>[2x]PGMAGDSEQTLQNHQQPNGGEPFLIGVSGGTASGKSSVCAKIVQLLGQNEVDYRQKQVVILSQDSFYRVLTSE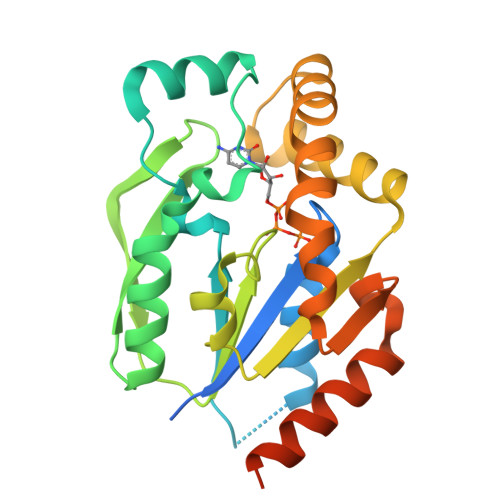QKAKALKGQFNFDHPDAFDNELILKTLKEITEGKTVQIPVYDFVSHSRKEETVTVYPADVVLFEGILAFYSQEVRDLFQMKLFVDTDADTRLSRRVLRDISERGRDLEQILSQYITFVKPAFEEFCLPTKKYADVIIPRGADNLVAINLIVQHIQDILNGGPSKRQTNGCLNGYTPSRK>LAKRIDAALILKDGRVVKGSNFENLRDSGDPVELGKFYSEIGIDELSFWDITASVEKRKTMLELVEKVAEQIDIPITVGGGIYDFETASELILRGAD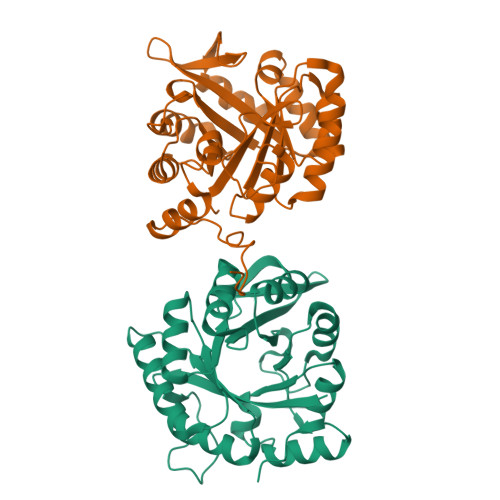KVEINTAAVENPSLITQIAQTFGSQAVVVYIAAKRVDGEFMVFTYSGTKNTGILLRDWVVEVEKRGAGEIVLGSIDRLGTKSGYDTEMIRFVRPLTTLPIIAHRGAGKTEHFLEAFLAGADAAKADSVFHSREIDVRELKEYLKKHGVNVRLEGLGSLEHHHHHH[2x]>GADGNEDLRADDLPGPAFESYESMELACPAERSGHVAVSDGRHMFVWGGYKSNQVRGLYDFYLPREELWIYNMETGRWKKINTEGDVPPSMSGSCAVCVDRVLYLF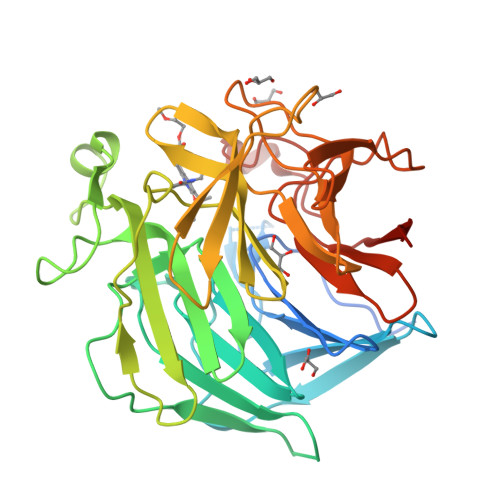GGHHSRGNTNKFYMLDSRSTDRVLQWERIDCQGIPPSSKDKLGVWVYKNKLIFFGGYGYLPEDKVLGTFEFDETSFWNSSHPRGWNDHVHILDTETFTWSQPITTGKAPSPRAAHACATVGNRGFVFGGRYRDARMNDLHYLNLDTWEWNELIPQGICPVGRSWHSLTPVSSDHLFLFGGFTTDKQPLSDAWTYCISKNEWIQFNHPYTEKPRLWHTACASDEGEVIVFGGCANNLLVHHRAAHSNEILIFSVQPK[2x]> GPGSDDEINAQS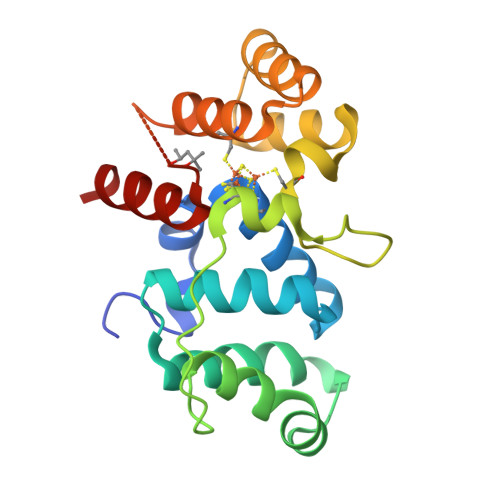VWSEEISSNYPLCIKNLMEGLKKNHHLRFFGRQQLSLFLKGIGLSADEALKFWSEAFTRNGNMTMEKFNKEFRFSFRHNYGLEGNRINFKPWDCHTILSKPRPGRGDFHGCPFRDWSHERLSAELRSMKLTQAQIISVLDSCQKGEYTIACTKVFEMTHNSASADLEIGEQTHIAHPNLYFERSRQLQK> MNQETLIAVVEQMRKLVPALRKVPDETLYAWVEMAELFVCQKTFKDAYVKALALYALHLAFLDGALKGEDEDLESYSRRVTSFSLSGEFSQTFGEVTKNQSGDMMLSTPWGKMFEQLKARRRGRF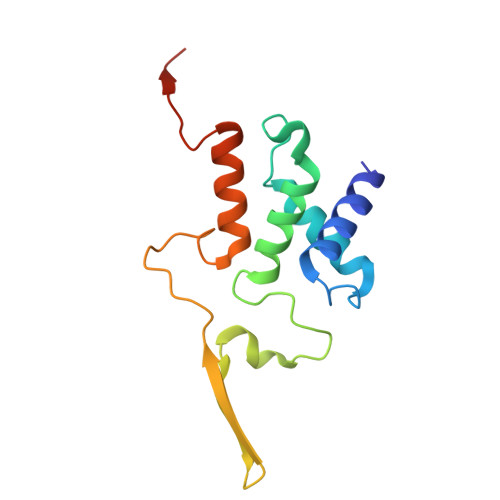ALMTGLRGGCH>[2x]MRIVAADTGGAVLDESFQPVGLIATVAVLVEKPYKTSKRFLVKYADPYNYDLSGRQAIRDEIELAIELAREVSPDVIHLDSTLGGIEVRKLDESTIDALQI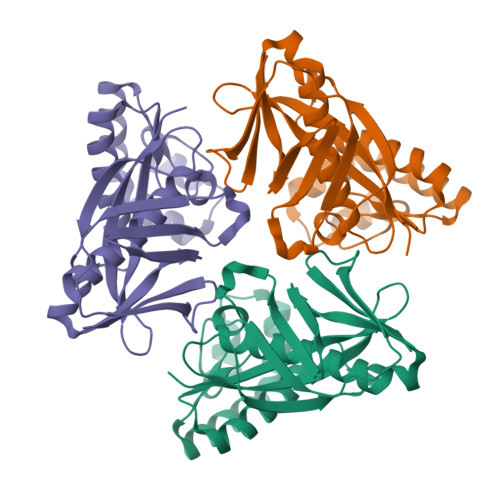SDRGKEIWKELSKDLQPLAKKFWEETGIEIIAIGKSSVPVRIAEIYAGIFSVKWALDNVKEKGGLLVGLPRYMEVEIKKDKIIGKSLDPREGGLYGEVKTEVPQGIKWELYPNPLVRRFMVFEITSKS>[4x]MNHKVHHHHHHMELGTLEGSRKQSKENTITINCVTFPHPDTMPEQQLLKPTEWSYCDYFWADKKDPQGNGTVAGFELLLQKQLKGKQMQKEMSEFIRERIKIEEEYAKNLAKLSQNSLAAQEEGSLGEAWAQVKKSLADEAEVHLKFSAKLHSEVEKPLMNFRENFKKDMKKCDHHIADLRKQLASRYASVEKARKALTERQKDLEMKTQQL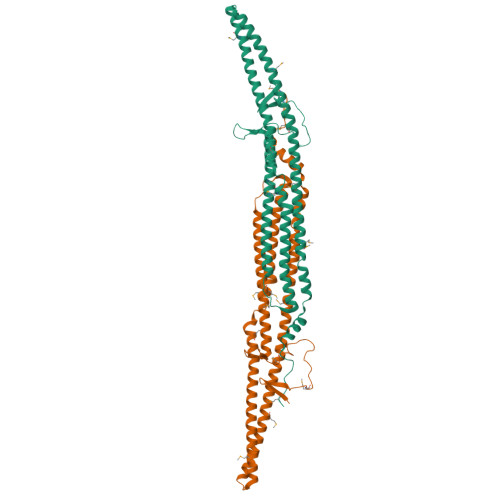EIKLSNKTEEDIKKARRKSTQAGDDLMRCVDLYNQAQSKWFEEMVTTTLELERLEVERVEMIRQHLCQYTQLRHETDMFNQSTVEPVDQLLRKVDPAKDRELWVREHKTGNIRPVDMEI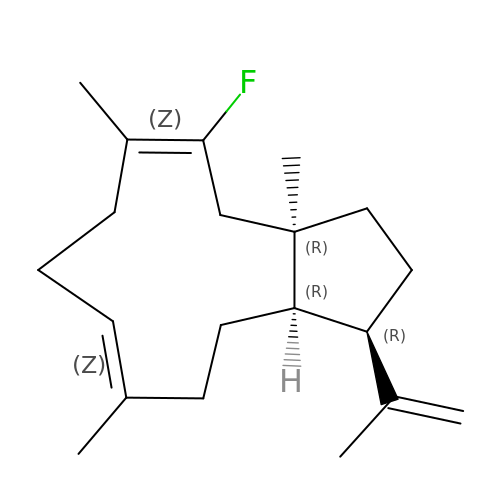2-fluoro-3,7,18-dolabellatriene | C20 H31 F | WCSSNSDHTDBDFK-PWWCRXLASA-N> GGGHMAKIIVKKSNPLKGSVKIDGAKNAVLPIIAATLLANGKSTLNGVPNLRDVHVISDLLRHVGAEVEYKENTLTVDASNIKTCEAPYELVRKMRASFLVMGPLLARFNSTKISMPGGSAIGTRPIDLHLKGFKALGAKIEMDHGFVEAATE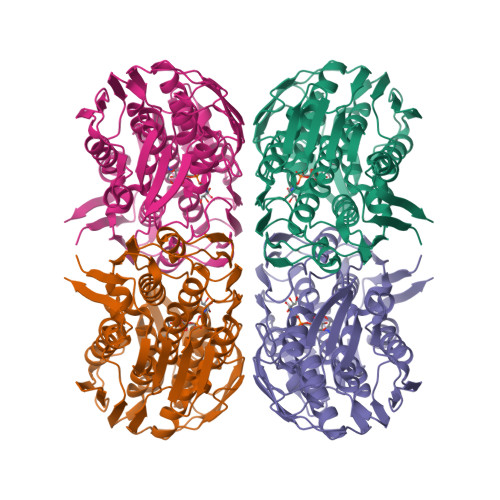KLVGNKLYLDFPSVGATENIMMAASLAEGTTIIENAAEEPEIVDLANFLNEMGADVKGAGTNTIKIKGVKELKGAEHNVIPDRIEAATYMVAAAMTKGDITVENVLMEHLKPVVAKLREAGCEITEMDNSVRVVGPKVLKPIDIKTLPHPGFPTDVQAQFMAMLTVANGTGVVIETVFENRFMHVAEFNRMGANIKIDGRSAVVNGVDELHGAAVNATDLRAGAALILCGLIAEGETQIGEIYHIQRGYVDIDKKITALGGQIEIVED>[4x]MRGSHHHHHHGLVPRGSKGTEEKQDSVRENLDKMISEAEVLNDMAARKLITLDAEQQLELMKSLVATQSQL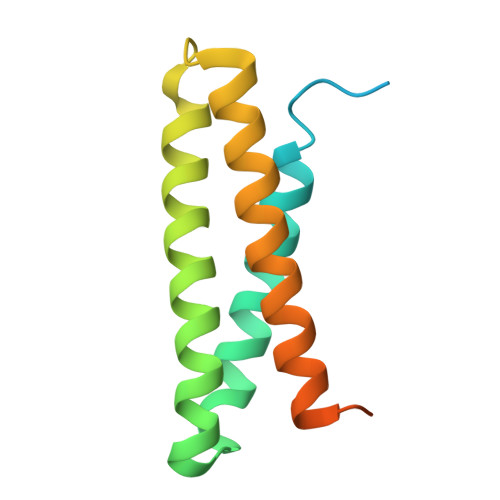EATKNLIGDPNATVADLQIAYTTLGNNTQALGNELIKLNPNGQIYAVLNNTEASRAATLRS> MADGMFAMPG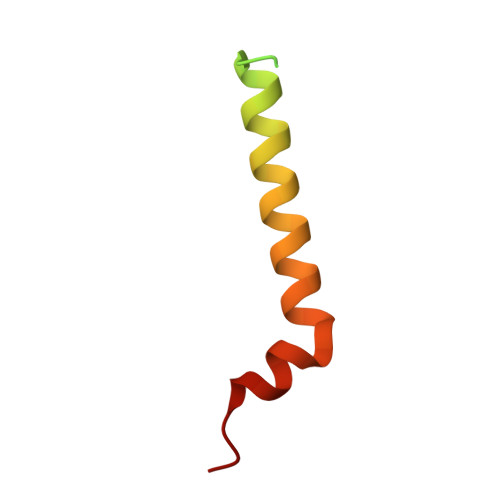AAAGAASPQQPKSRFQAFKESPLYTIALNGAFFVAGVAFIQSPLMDMLAPQL> NCDIVIVGGGSAGSLLAARLSEDPDSRVLLIEAGEEPTDPDIWNPAAWPALQGRSYDWDYRTEAQAGTAGRAHHWARGRLIGGSSCLHAMGYMRGHPSDFQAWVDASGDRRWGWDELLPVFQAIEDHPLGGDGIHGKGGPLPIHLPADEVSPLARAFIEAGASLGLPRLEGHNSGEMIGVTPNSLNIRDGRRVTAADAWLTKAVRGRKNLTILTGSRVRRLKLEGNQVRSLEVVGRQGSAEVFADQIVLCAGALESPALLMRSGIGPHDVLDA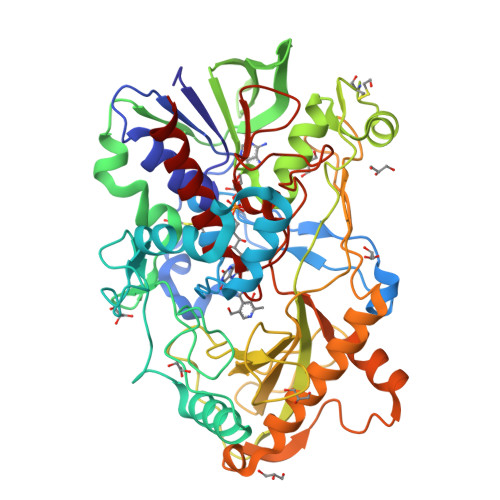AGVGCLIDMPDIGRNLQDHLLGAGNLYAARKPVPPSRLQHSESMAYMRADSFTAAGQPEIVVGCGVAPIVSESFPAPAAGSAYSLLFGITHPTSRGSVRISGPELGDRLIIDPAYLQTGRDRERFRRALEASRTIGHRDELAGWRERELLPGTPNSAAEMDDFIARSVITHHHPCGTCRMGKDPDAVVDANLRLKALDNLFVVDASIMPNLTAGPIHAAVLAIAETFARQYHHHH> QVDMLLQEMADEAGLDLN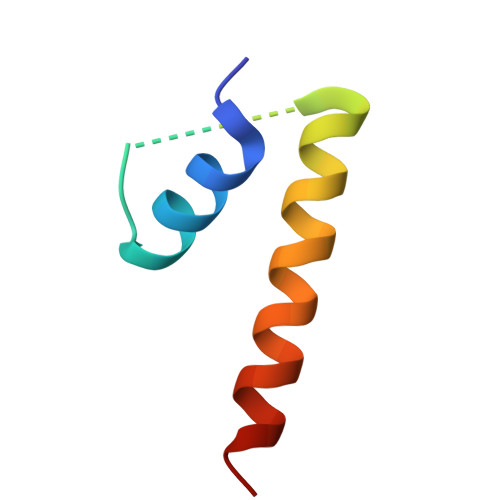MELPQGQTGSVGTSVASAEQDELSQRLARLRD>[8x]MIWKRKITLEALNAMGEGNMVGFLDIRFEHIGDDTLEATMPVDSRTKQPFGLLHGGASVVLAESIGSVAGYLCTEGEQKVVGLEINANHVRSAREGRVRGVCKPLHLGSR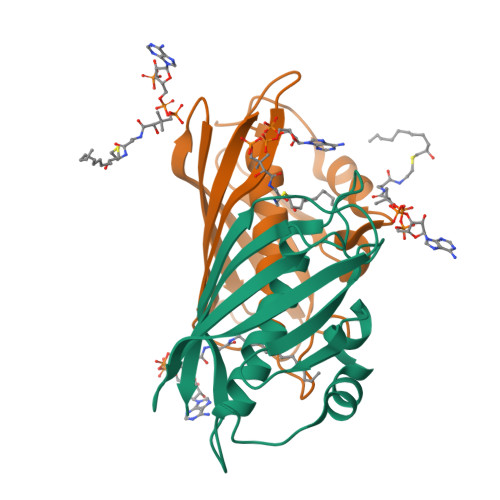HQVWQIEIFDEKGRLCCSSRLTTAIL There has been considerable interest towards an improved understanding of the cleavage mechanisms that underlie RNA catalysis by small self-cleaving ribozymes involved in self-scission during rolling circle replication of viral genomes. Such challenges are highlighted by the recent identification of a new set of self-cleaving ribozymes from genomic bioinformatics searches, named twister, twister-sister, pistol, and hatchet ribozymes. We report here the structure of a four-way junctional twister-sister ribozyme and discuss possible/putative roles of selected nucleobases and hydrated Mg2+ ions observed at the active site for cleavage chemistry. For crystallographic studies, we introduced dC62 into the sequence of the longer substrate strand of the two-stranded construct, so as to prevent cleavage at the known C62–A63 cleavage site of the twister-sister ribozyme.

We have identified a large number of hydrated Mg2+ cations distributed throughout the tertiary fold of the twister-sister ribozyme (green balls), with divalent cation Mg2+ occupancy confirmed followed substitution by Mn2+ and monitoring the latter’s anomalous diffraction characteristics. We have undertaken Mn2+ soak experiments to use the anomalous properties of these ions to definitively differentiate between monovalent and divalent cation sites. These experiments (examples shown for M1 to M7 in Supplementary Fig. 4b–g) unambiguously establish that M1 to M7 are all divalent cations, with the observed octahedral geometry for M1 to M7 with metal to water oxygen distances of 2 Å, consistent with hydrated Mg2+ for these metal sites (M1–M4 are shown in Fig. 3c–e; M5 is shown in Fig. 2a and b, and M6–M7 are shown in Fig. 2e and g). In addition, U36 forms extensive interactions with G59 and the A8–G9 step through two hydrated Mg2+ cations M6 and M7, which were confirmed by the anomalous signal collected with Mn2+-soaked crystals. Interestingly, one metal designated as M8, that is coordinated to N7 of G35 has strong anomalous signal in the Mn2+-soaked crystals, whereas its counterpart is not observed in the native crystal, which may explain why the three-stranded native twister-ribozyme construct has better cleavage activity with Mn2+ than Mg2+ under 2 mM divalent cation conditions.

>ACCCGCAAGGCCGACGGC[2x];>[2x]GCCGCCGCUGGUGCAAGUCCAGCCACGCUUCGGCGUGGGCGCUCAUGGGU> GPAGSMATERDQEIIDFIDQGNYTYAQSLITKKLAKSPQKLFYHVLQNEIHLKSGQRELAIKKNLELLNRYPNDPLTIEKLSDFFSKMEMEKESSLVYENAIKKYPVSTETLCLSWFDNSIEKYDFKVFNRIFMYLNKNGKSRLHTLWYAFSFHLLLQEGETDKASLYNSLGKKLMEGLQPFENTQEIYVYTLFLSSKEIEQVLSGVTLPLDLELKLLYMKAMKENASFEALHAYTEKLLFKEKFDDFDTWKLWILSGKEIGKSFEELDQKLTLPTRNISLLKIELDILYSRNIETSVENYYQKFNTKLCCYADLSQYELPTSFIGSLKNSTSEENLITVVNNRKFVNQTDNWDVYERFSTKEGAEYDSNPVNELTLR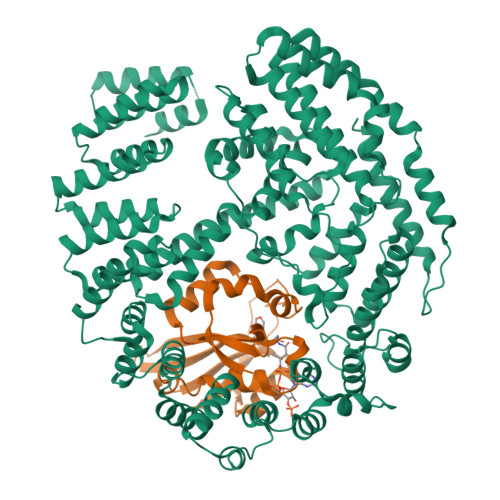TIVSDLDSSPQNTIKNIVLLKHLLEQDKYNYKLKLWLMKLYSQLNTNDLIFPIYNGLKIRMTQHETLNYYLTTTNPSKINLDAWVDIYRFYLTSKQEIKESIIQGFDNGVFNKLEGFINFSKRMQNSISLNFTVAKILQISTILGTDGYLNYFIHYLKTNEALIVSDYTDNRDFKSEWNGLEKIDCIDVPVNDVATKLKLLVYSIVFEDQDASRLLKVFNKITSNAKFSVFDNLLYKLYFNLLKITKTKLNPQETQSLYNYLQKNLKTDKLKILIPENLLSGELTQNLTNLVEFIKIVKLLAKRHPSSYMNQLVNLVKPFGKEFKNLKLVQRQHEIIDSMDFEPPISVDISQTKLEIKSSIEDCVVALLNSL;> MTSIKPFQMEDLFELNPVNLDPLTENFNVSFYSQYLIEWPQLFYKSVETPNGQASGYMMAKTEGQLSKKEWHTHITAVTVLDQYRRIGLASKLCLELENLTQVKDTLFIDLFVKVTNTLGRILYEKLGYSVFRRVVGYYGREIQKDRNKIDDSVDAFDMRKLLPRDVNNE>[2x]MYGLVNKAIQDMISKHHGEDTWEAI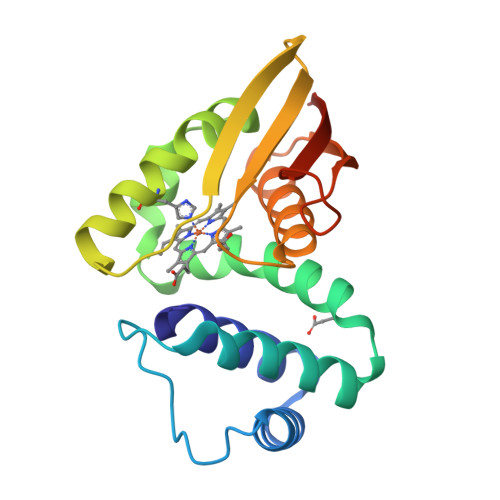KQKAGLEDIDFFVGMEAYSDDVTYHLVGAASEVLGKPAEEWWIAFGEYWVTYTSEEGYGELLASAGDSLPEFMENLDNLHARVGLSFPQLRPPAFECQHTSSKSMELHYQSTRCGLAPMVLGLLHGLGKRFQTKVEVTQTAFRETGEDHDIFSIKYEDSNLYDD3-CYCLOPENTYL-N-HYDROXYPROPANAMIDE 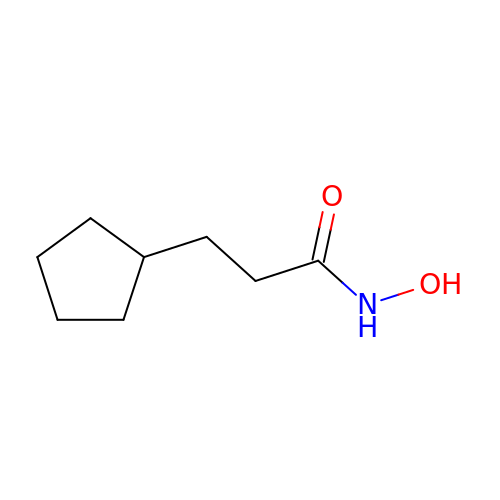| C8 H15 N O2 | PCDWXHSMVLWAMG-UHFFFAOYSA-N> GPDDPLVINGEIEIVTRAPTPAHLADRFDEIRSGWTFRTDDTQALEMDDFENSGMVFVEEARAVWDRPEGTEGKACADCHGAVDDGMYGLRAVYPKYVESAGKVRTVEQMINACRTSRMGAPEWDYIGPDMTAMVALIASVSRGMPVSVAIDGPAQSTWEKGREIYYTRYGQLDLSCASCHEQYFDHYIRADHLSQGQINGFPSYRLKNARLNAVHDRFR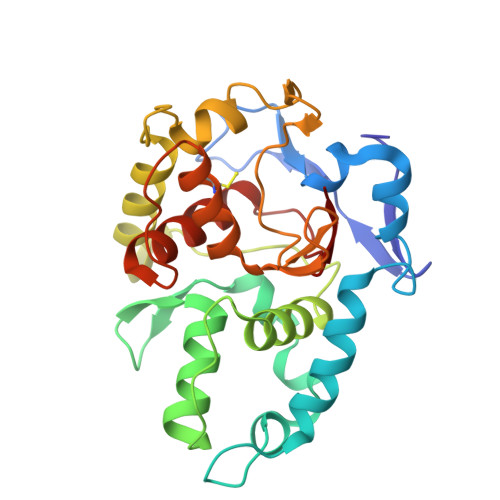GCIRDTRGVPFAVGSPEFVALELYVASRGNGLSVEGPSVRN> 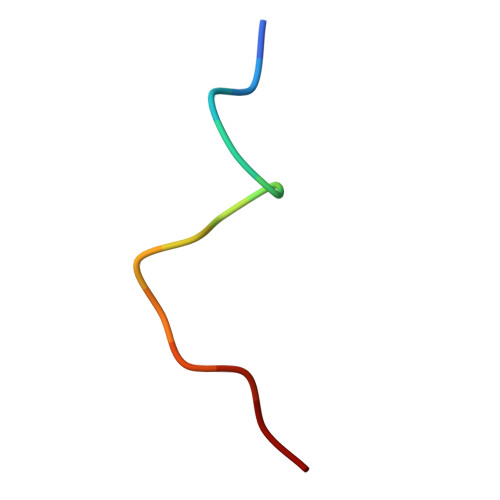ATGAGAGAGTTPGP>[2x]MNYPVN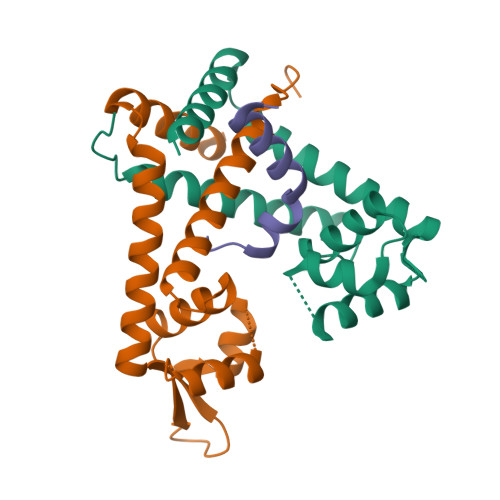PDLMPALMAVFQHVRTRIQSELDCQRLDLTPPDVHVLKLIDEQRGLNLQDLGRQMCRDKALITRKIRELEGRNLVRRERNPSDQRSFQLFLTDEGLAIHLHAELIMSRVHDELFAPLTPVEQATLVHLLDQCLAAQ;> RRDYTEQLRRAARRNAWDLYGEHFY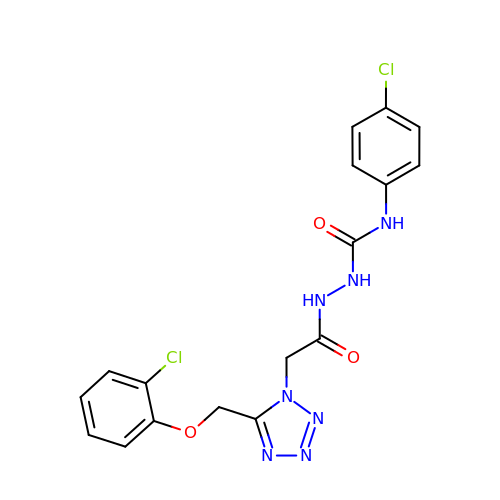2-({5-[(2-chlorophenoxy)methyl]-1H-tetrazol-1-yl}acetyl)-N-(4-chlorophenyl)hydrazinecarboxamide | C17 H15 Cl2 N7 O3 | ZWKKYQAZABDTRS-UHFFFAOYSA-N> MKNCVIVSAVRTAIGSFNGSLASTSAIDLGATVIKAAIERAKIDSQHV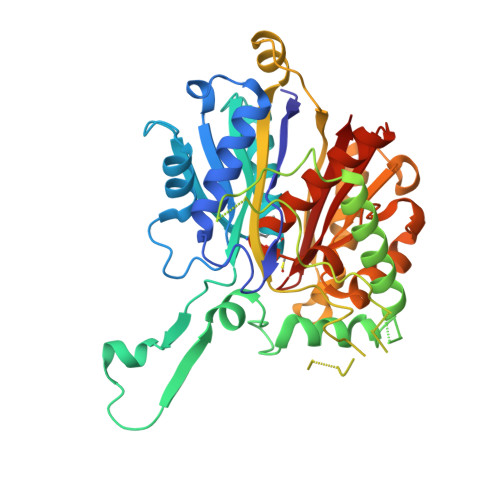DEVIMGNVLQAGLGQNPARQALLKSGLAETVCGFTVNKVCGSGLKSVALAAQAIQAGQAQSIVAGGMENMSLAPYLLDAKARSGYRLGDGQVYDVILRDGLMCATHGYHMGITAENVAKEYGITREMQDELALHSQRKAAAAIESGAFTAEIVPVNVVTRKKTFVFSQDEFPKANSTAEALGALRPAFDKAGTVTAGNASGINDGAAALVIMEESAALAAGLTPLARIKSYASGGVPPALMGMGPVPATQKALQLAGLQLADIDLIEANEAFAAQFLAVGKNLGFDSEKVNVNGGAIALGHPIGASGARILVTLLHAMQARDKTLGLATLCIGGGQGIAMVIERLN> SLKLFLFEFATCGERIEDSTAVEGLAMFKSAFDGFKNYYEITGFVRPEFSCLFTLPVDSMDSMEKYLEKSDAFLIIAPEDDFLLYTLTKKAEKYCEN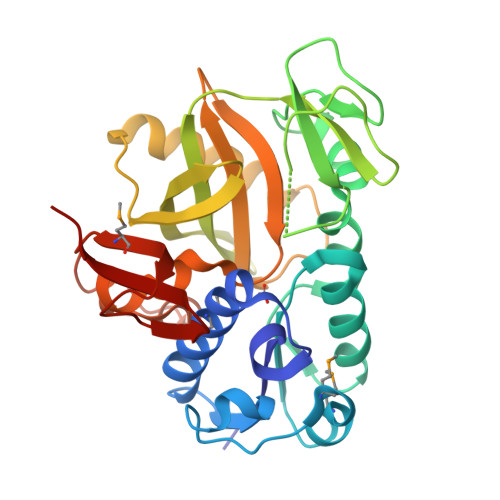LGSSSRAIAVTSDKWELYKKLRGEVQVPQTSLRPLDCKFIIKPRTACAGEGIGFSDEVPDGHIAQEFIEGINLSVSLAVGEDVKCLSVNEQIINNFRYAGAVVPARISDEVKREVVEEAVRAVECVEGLNGYVGVDIVYSDQPYVIEINARLTTPVVAFSRAYGASVADLLAGGEVKHVRRQMVRKSKSAEKPYVSVGDYTLEIIDLD>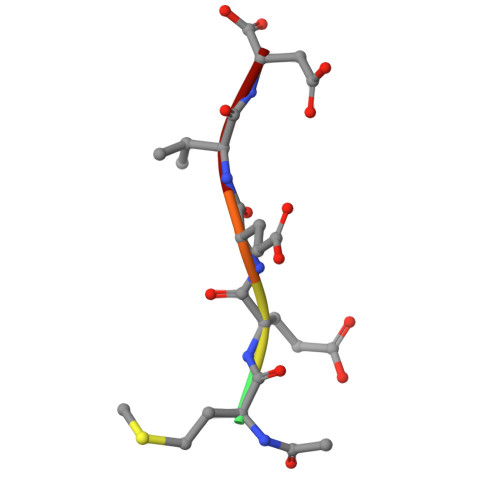 XMEEVD> GAV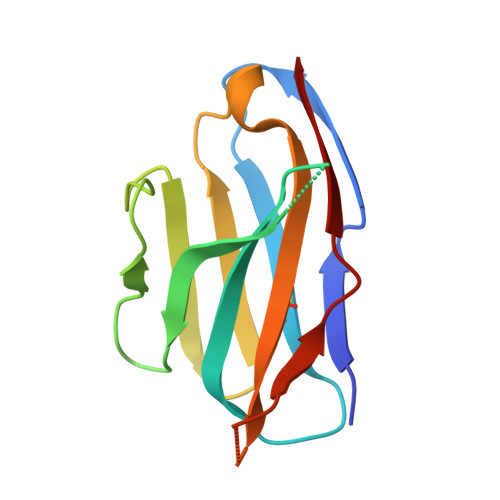VSQHPSRVIVKSGTSVKIECRSLDFQATTMFWYRQFPKQSLMLMATSNEGSKATYEQGVEKDKFLINHASLTLSTLTVTSAHPEDSGFYICSALAGSGSSTDTQYFGPGTRLTVL>[6x]MTSAEMTSPNNNSEHQAIAKMRTMIEGFDDISHGGLPIGRSTLVSGTSGTGKTLFSIQFLYNGIIEFDEPGVF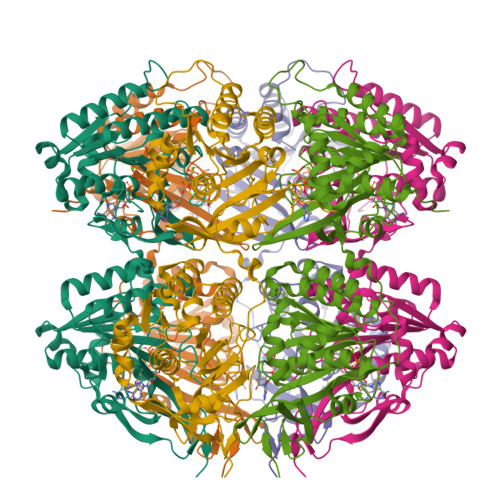VTFEETPQDIIKNARSFGWDLAKLVDEGKLFILDASPDPEGQEVVGGFDLSALIERINYAIQKYRARRVSIDSVTSVFQQYDASSVVRRELFRLVARLKQIGATTVMTTERIEEYGPIARYGVEEFVSDNVVILRNVLEGERRRRTLEILKLRGTSHMKGEYPFTITDHGINIFPLGAMRLTQRSSNVRVSSGVVRLDEMCGGGFFKDSIILATGATGTGKTLLVSRFVENACANKERAILFAYEESRAQLLRNAYSWGMDFEEMERQNLLKIVCAYPESAGLEDHLQIIKSEINDFKPARIAIDSLSALARGVSNNAFRQFVIGVTGYAKQEEITGLFTNTSDQFMGAHSITDSHIEAITDTIILLQYVEIRGEMSRAINVFKMRGSWHDKAIREFMISDKGPDIKDSFRNFERIISGSPTRITVDEKSELSRIVRGVQEKGPES>[2x]MAHHHHHHMNLSTPRPIEERTGAPDWDRVRLDFPLLMREVHGKPLVYFDNANTGQKPVQVIGAVDEFYRRYNANVSRAVHALGSEATDAYEGARNTLARFLNVRPSDLVLCSGTTFAINLVAYSWALPRLKAGDVILITRMEHHANIVPWQLVAQRTGATIRVAEITPD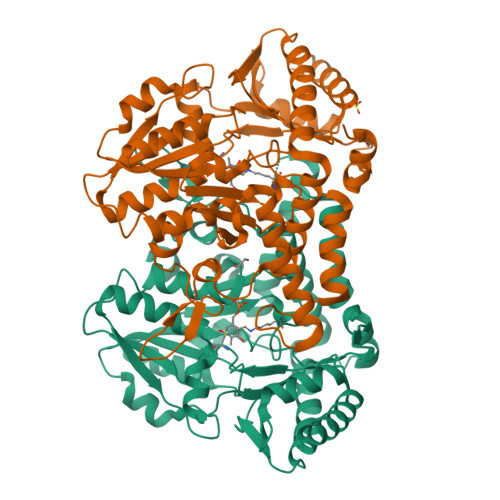GALDLDALRAAMTPEVKLLAVTHVSNVLGTVNPVREICREARKRGIITVVDGSQAVPHRKVDVAAIGCDFYAITGHKMCGPTGTGALWARREHLDAMPPFLGGGEMIKEVSFDGTVFNDAPHKFEAGTPNIAGFIGLGVAADYLQQLGQENVEAREAELLAHFTEELRRVDGLRIIGEAPEKAAVVSFLIDGAHAHDLATLLDLEGVAVRSGQHCAHPLLQYFGVAATCRASLAFYNTHAEIERFMTALTKVRKLLG[9-[2-carboxy-5-[2-[2-[4-(trifluoromethylsulfonylamino)butoxy]ethoxy]ethylcarbamoyl]phenyl]-6-(dimethylamino)xanthen-3-ylidene]-dimethyl-azanium 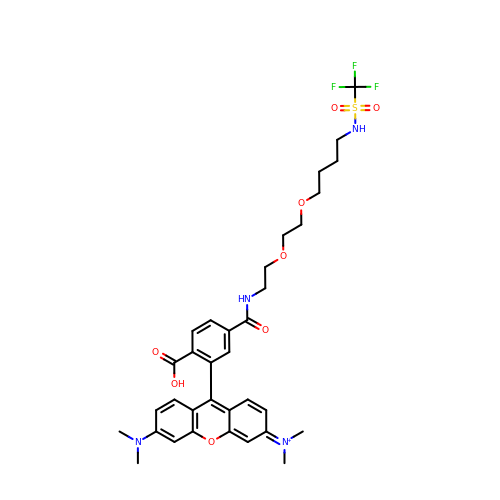| C34 H40 F3 N4 O8 S | CKSQAQHVRBNIHM-UHFFFAOYSA-O>[2x]MAKNTITKTLKLRIVRPYNSAEVEKIVADEKNNREKIALEKNKDKVKEACSKHLKVAAYCTTQVERNACLFCKARKLDDKFYQKLRGQFPDAVFWQEISEIFRQLQKQAAEIYNQSLIELYYEIFIKGKGIAN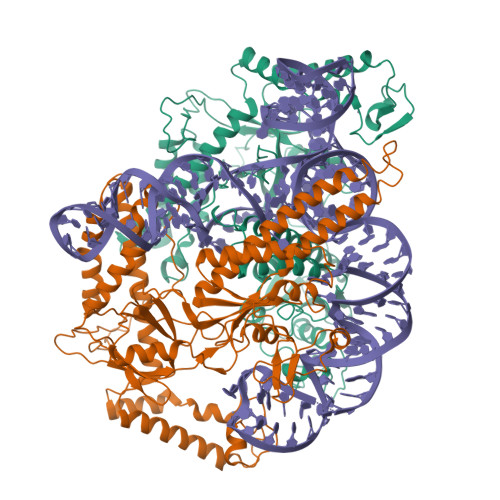ASSVEHYLSDVCYTRAAELFKNAAIASGLRSKIKSNFRLKELKNMKSGLPTTKSDNFPIPLVKQKGGQYTGFEISNHNSDFIIKIPFGRWQVKKEIDKYRPWEKFDFEQVQKSPKPISLLLSTQRRKRNKGWSKDEGTEAEIKKVMNGDYQTSYIEVKRGSKICEKSAWMLNLSIDVPKIDKGVDPSIIGGIDVGVKSPLVCAINNAFSRYSISDNDLFHFNKKMFARRRILLKKNRHKRAGHGAKNKLKPITILTEKSERFRKKLIERWACEIADFFIKNKVGTVQMENLESMKRKEDSYFNIRLRGFWPYAEMQNKIEFKLKQYGIEIRKVAPNNTSKTCSKCGHLNNYFNFEYRKKNKFPHFKCEKCNFKENADYNAALNISNPKLKSTKEEP> RFESVALEQ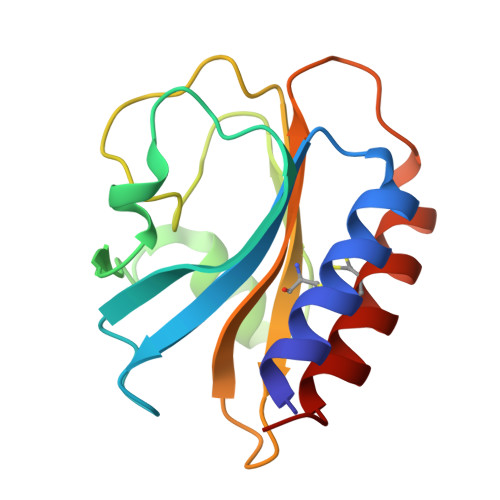LQIVHISSEADFSAVYSFRPKNLNYFVDIIAYEGKLPSTISEKSLGGYPVDKTMDEYTVHLNGRHYYSNSKFAFLPTKKPTPEINYMYSCPYFNLDNIYAGTITMYWYRNDHISNDRLESICAQAARILGRAK> DYKDDDDKALSLLLFVANRPGDEEETAAIQAHIQQLPSNFSFELKVVPIGEQPYLLEEYKLVATPALIKVRPEPRQTLAGRKLLQKVDYWWPRW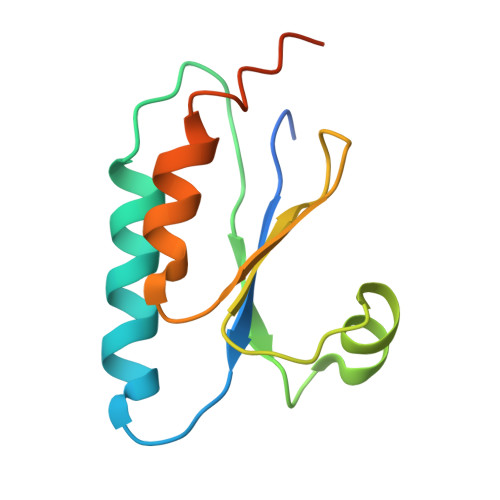QREVALDYKDDDDK O1-tert-butyl O2-ethyl 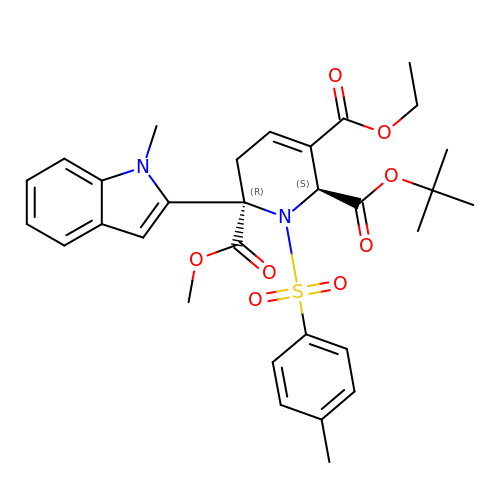O5-methyl (E,5R)-5-(1-methylindol-2-yl)-5-[(4-methylphenyl)sulfonylamino]pent-2-ene-1,2,5-tricarboxylate | C31 H36 N2 O8 S | FUSYRUNCXNWFDD-SUYBVONHSA-N> GTSRRLSLFFSDPPPAYALSLHAGYKIQAALCVDRLPLVYREPRYEKRWREFKEQWEAQTKNGLTLADEITFMKFPFHFFETEEAQKKREELISKTGDAEVSELELLLSEEGFSGKRKLQRDRDAKKAAREEQSAVKSAGRGQDEKGLRSLEREPERTLYLIVRYGDSWQFPLEDRIHG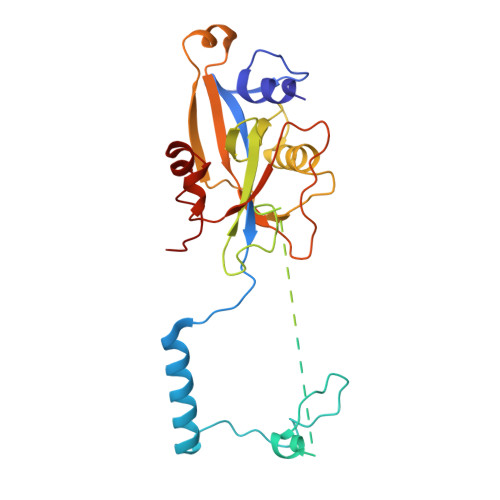QSMRSTLKRLCSEQLGSSYAPFLLGYSPFSYAKRTYPKKTKEAGILGRKIFYYRAHHIPGSENLKLPEGSPVSDFAWVTLQELPAYISPRKLAAVSAGLLLEE> QECSLQSCTQHQPYVVDDPCPIHFYSKWYIRVGARKSAPLIELCVDEAGSKSPIQYIDIGNYTVSCSPFTINCQEPKLGSLVVRCSFYEDFLEYHDV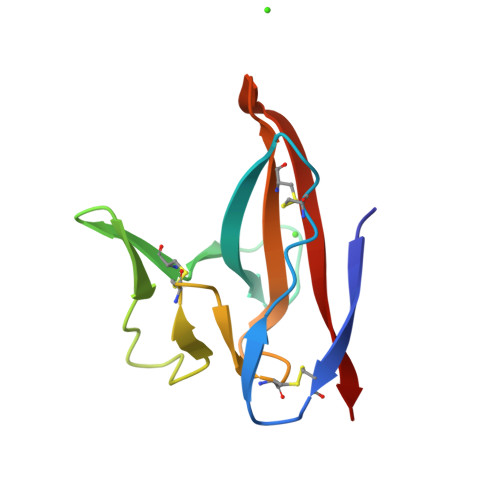RVVLDFI>[2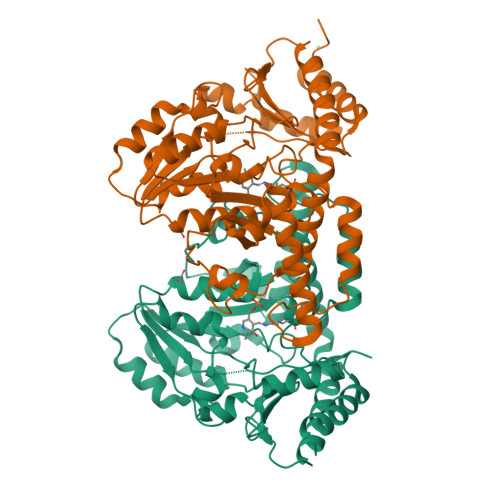x]MAHHHHHHMIYLDHNATTFIDPRVKEFIISLMDKELNPSSAHSSGRFAKNLIETVRAQIATALGITLSSREYDITFTSSGTEGNNLIMKNFYDGDIFISAIEHLSIYNHINYAPNIKVISVNTQGLVDLEHLEELLAQSNTSKKLVSIIMANNESGVLQDIAEIGKITKKYEAKFHSDLVQGFGRIPINIKALGLDFATISGHKIGGGQGGAALISSSNFQITPMIIGGGQEKSVRSGTENVLAIAGFGLASALRTDNISENYIKIKKLQENLEKKLKKYPNVNIVSNNVARLPNTTLITIPNTDAQAKLIGFDLHNICVSSGSACSSGKISKSHVLTNMGVGEEEAKSSIRISLSHTNTVRDIEAFIEAFEEIYDVIPS>MTNSSASQKKRSKGSAQDWHRAD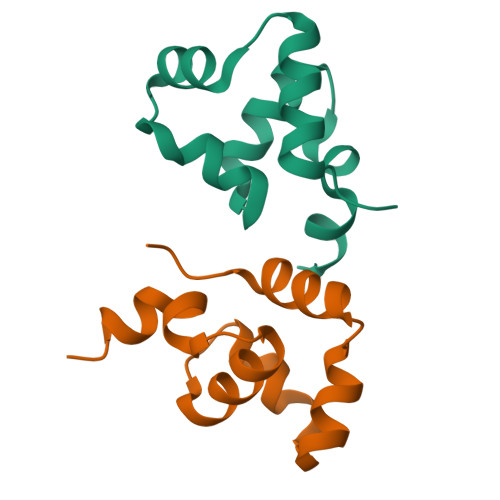IVAALHKRGITLAGLSRAHGLAARTLSNAMERHYPRAERLIAQALDMRPEDIWPQRYRNKKTDGEKE[2x]> ASSTNLKDVLAALIPKEQARIKTFRQQHGGTALGQITVDMSYGGMRGMKGLVYETSVLDPDEGIRFRGFSIPECQKLLPKGGGGEPLPEGLFWLLVTGQIPTGAQVSWLSKEWAKRAALPSHVVTMLDNFPTNLHPMSQLSAAITALNSESNFARAYAEGILRTKYWEMVYESAMDLIAKLPCVAAKIYRNLYRAGSSIGAIDSKLDWSHNFTNMLGYTDAQFTELMRLYLTIHSDHEGGNVSAHTSHLVGSALSDPYLSFAAAMNGLAGPLHGLANQEVLGWLAQ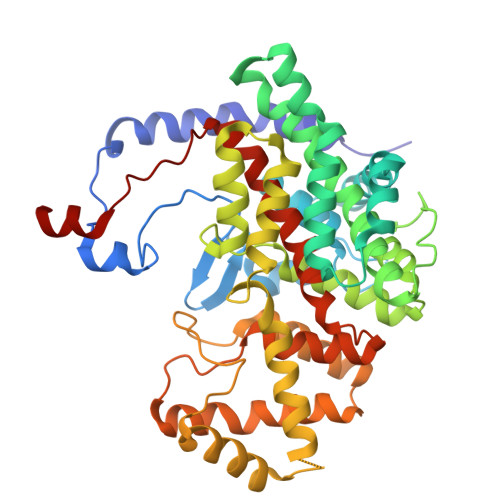LQKAAGADASLRDYIWNTLNSGRVVPGYGHAVLRKTDPRYTCQREFALKHLPGDPMFKLVAQLYKIVPNVLLEQGAAANPWPNVDAHSGVLLQYYGMTEMNYYTVLFGVSRALGVLAQLIWSRALGFPLERPKSMSTDGLIAL2-BROMO-6-HYDROXY-PURINE | C5 H3 Br 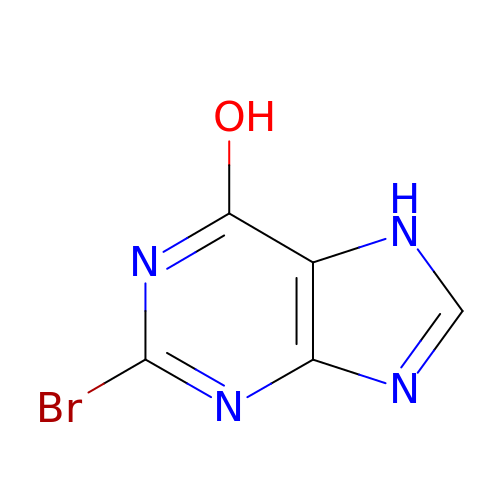N4 O | ONXCBJOMYNPZNI-UHFFFAOYSA-N>[2x]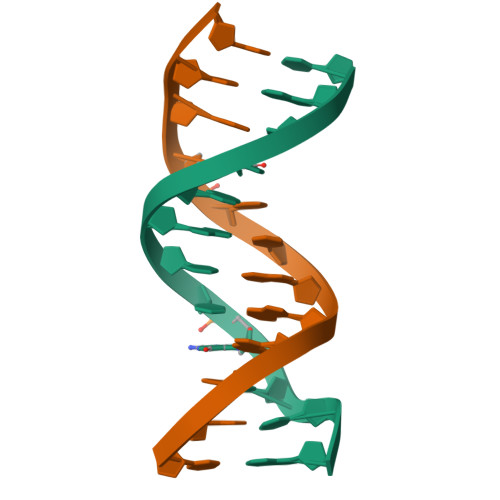CGCAAATTGGCG(2~{S})-2-[2-[4-(4-methoxyphenyl)phenyl]sulfonylphenyl]pentanedioic acid | C24 H22 O7 S | 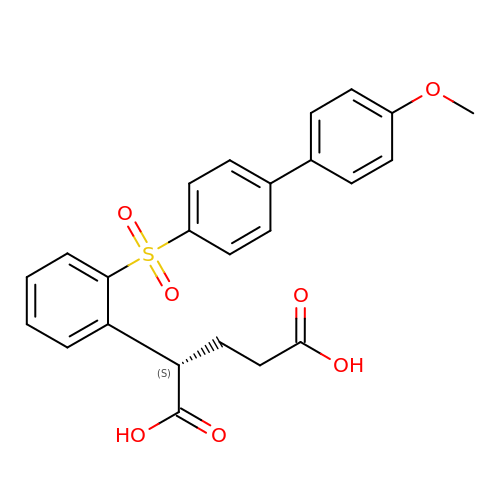QMSIXYWYTRVTIW-NRFANRHFSA-N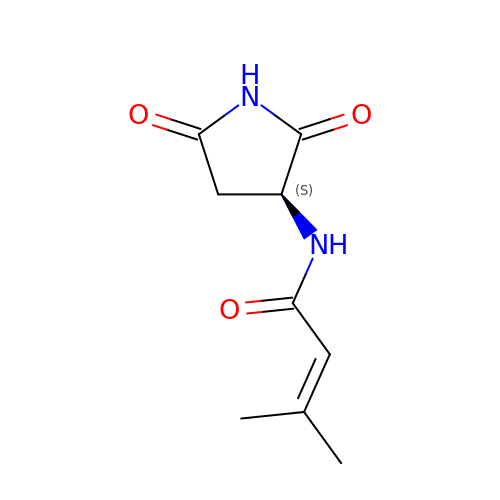~{N}-[(3~{S})-2,5-bis(oxidanylidene)pyrrolidin-3-yl]-3-methyl-but-2-enamide | C9 H12 N2 O3 | RSHQAELIOFFTCL-LURJTMIESA-N>MMKRNILAVIVPALLVAGTANAAEIYNKDGNKVDLYGKAVGLHYFSKGNGENSYGGNGDMTYARLGFKGETQINSDLTGYGQWEYNFQGNNSEGADAQTGNKTRLAFAGLKYADVGSFDYGRNYGVVYDALGYTDMLPEFGGDTAYSDDFFVGRVGGVATYRNSNFFGLVDGLNFAVQYLGKNERDTARRSNGDGVGGSISYEYEGFGIVGAYGAADRTNLQEAQPLGNGKKAEQWATGLKYDANNIYLAANYGETRNATPITNKFTNTSGFANKTQDVLLVAQYQFDFGLRPSIAYT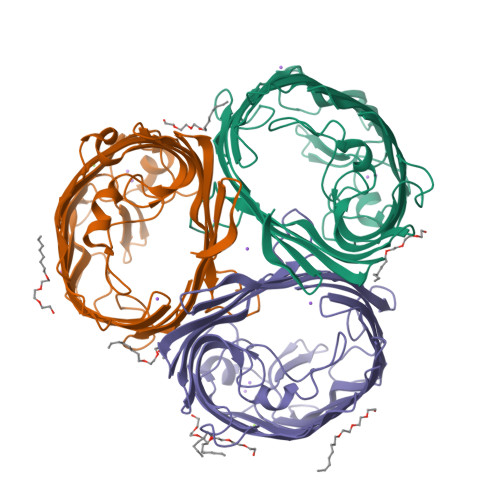KSKAKDVEGIGDVDLVNYFEVGATYYFNKNMSTYVDYIINQIDSDNKLGVGSDDTVAVGIVYQF[3x]>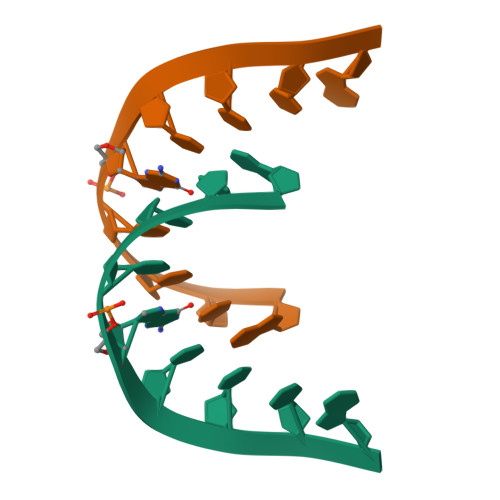 GCCUGCCUG> DIDQ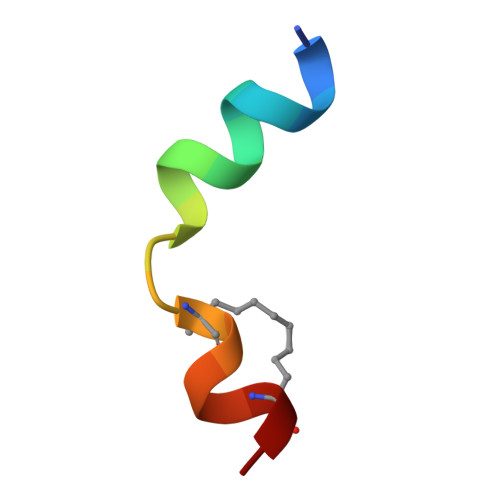MFSTLLGELDLLLQS>MNIHVTIREATEGDLEQMVHMLADDVLGRKRERYEKPLPVSYVRAFKEIKKDKNNELIVACNGEEIVGMLQVTF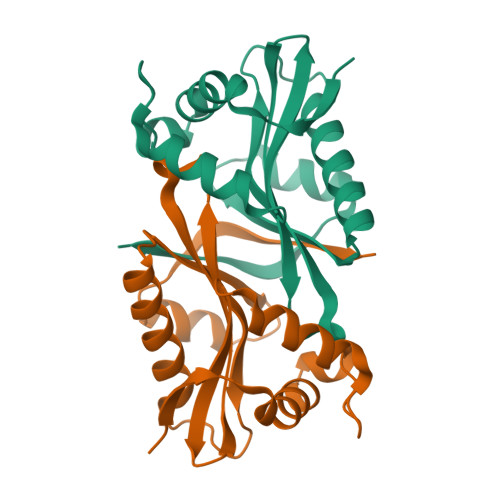TPYLTYQGSWRATIEGVRTHSAARGQGIGSQLVCWAIERAKERGCHLIQLTTDKQRPDALRFYEQLGFKASHEGLKMHF[2x]> EFMNAPLRGQVYRCDLGYGAKPWLIVSN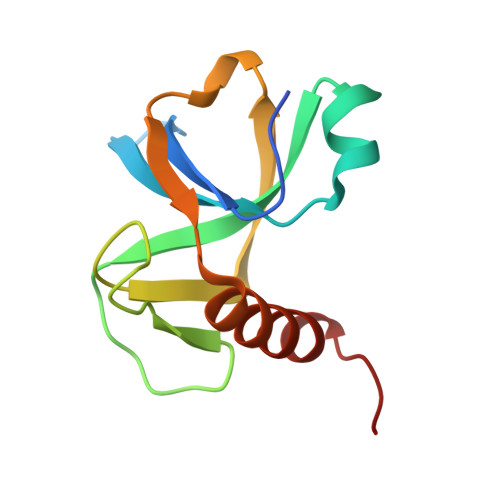NARNRHTADVVAVRLTTTRRTIPTWVAMGPSDPLTGYVNADNIETLGKDELGDYLGEVTPATMNKINTALATALGLPWP> GPLGSSKTNNLIVVSIDPMEYIYKPLTHA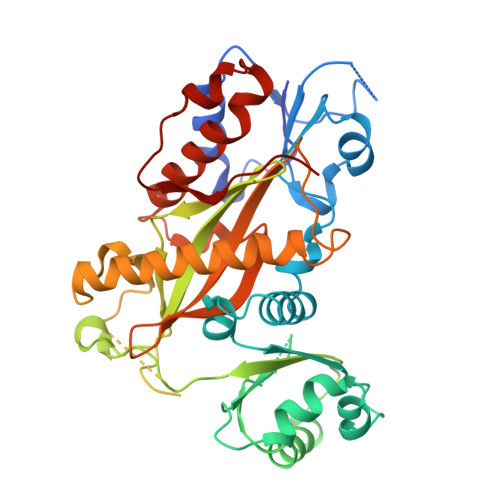LKKYLPQVEIVSNLPEFDNGGCEKEMKVFHYGDYEQLDMDKLMELPNNYFTNSYIYRKALIRKHFLSHTIQTYTAKNPESILKKAYLESFTIDLDYAEFLDDALDENWELRQELENESQDKWWIVKPSMSDKGQGIRVFKTIEDLQAIFDSFDDEDSEAEESGNDDDADDVNGEFMDNNKVNISQLRHFIIQEYLTNPLLLASMDNRKFHIRCYVVCRGDLQVFVYDRMLALFAAKPFVPLDPYAYSVTDLKDLECHLTNTCLQSKKKDKDSSVLEFDSIEEIPNERKSNIKEQIHSITNDVFLAAVNVNRLNFQPLPNAFETYGVDFLIDSNYEVKLLEINAFPDFKQTGKDLKNLIDELFDDTVKYCVTPIFNENRNKTDDETDPNFVKVIDYTSNGW> GMSRTNINFNNKRTELANKIWDIFIAN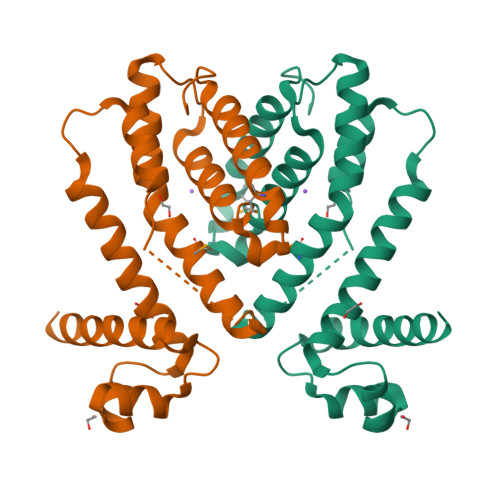GYENTTLAFIINKLGISKGALYHYFSSKEECADAAIENRVAFFSNEVLKESEEGLNSIERLKKILLAGIKITSVNEQVKEINSPSNKIFHQKLMVAIIKYFAPIYADIISQGNEEGVFKVKYPLETAEIILTLSHFYLDEDLFKWKKEDMSLKLTAFKETLIKILDADEDTFDFIK> EWTGDSSI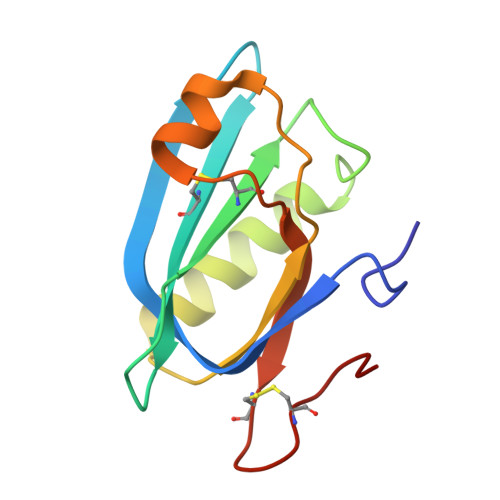NYYSDEVISDFHVGQFNRSAYFCIKTVKKSGEGTPIIACALSHDSKWIPSFNIMLEQARNFYITGHSIRVYVQPNVWSNKSFIEALSSNALVGLSSCSTSECFGPVKP>MASWSHPQFEKGGTHVAETSAPTRSEPDTRVLTLPGTASAPEFRLIDIDGLLNNRATTDVRDLGSGRLNAWGNSFPAAELPAPGSLITVAGIPFTWANAHARGDNIRCEGQVVDIPPGQYDWIYLLAASERRSEDTIWAHYDDGHADPLRVGISDFLDGTPAFGELSAFRTSRMHYPHHVQEGLPTTMWLTRVGMPRHGVARSLRLPRSVAMHVFALTLRTAAAVRLAEGATT[2x];>MGSSHHHHHHSQDPNSTTTAPPVELWTRDLGSCLHGTLATALIRDGHDPVTVLGAPWEFRRRPGAWSSEEYFFFAEPDSLAGRLALYHPFESTWHRSDGDGVDDLREALAAGVLPIAAVDNFHLPFRPAFHDVHAAHLLVVYRITETEVYVSDAQPPAFQGAIPLADFLASWGSLNPPDDADVFFSASPSGRRWLRTRMTGPVPEPDRHWVGRVIRENVARYRQEPPADTQTGLPGLRRYLDELCALTPGTNAASEALSELYVISWN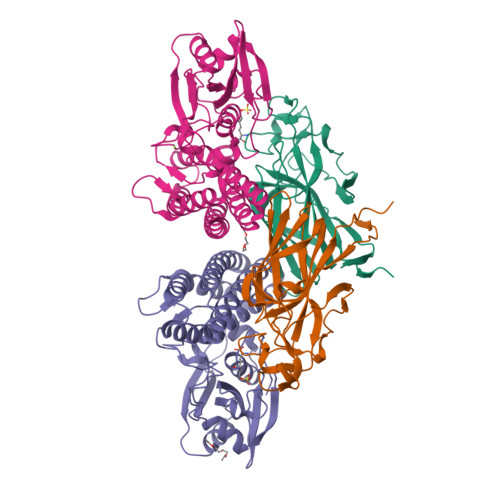IQAQSGLHAEFLRAHSVKWRIPELAEAAAGVDAVAHGWTGVRMTGAHSRVWQRHRPAELRGHATALVRRLEAALDLLELAADAVS[2x]> MQKLTVGLIGNPNSGKTTLFNQLTGARQRVGNWAGVTVERKEGIFATTDHQVTLVDLPGTYSLTTISSQTSLDEQIACHYILSGDADML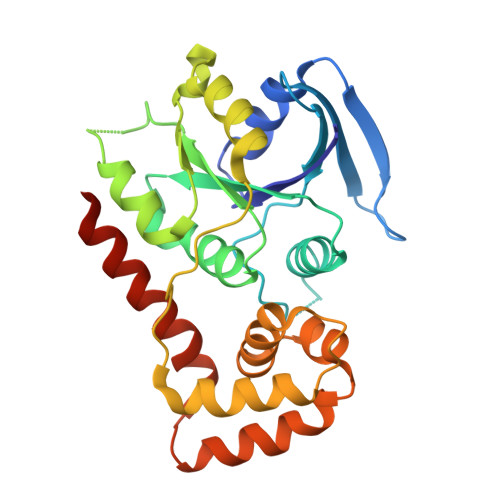INVVDASNLERNLYLTLQLLELGIPCVVALNMLDIAEKQQVRIDIDALAARLGCPVIPLVSTRGRGIEALKIALDRHQANSDLELVHYPQPLLREADLLAQQMSAQIPPRQRRWLGLQMLEGDIYSRAYAGDAADKLDIALANLSDEIDDPALHIADARYQTIAAICDAVSNTLTAEP> GHR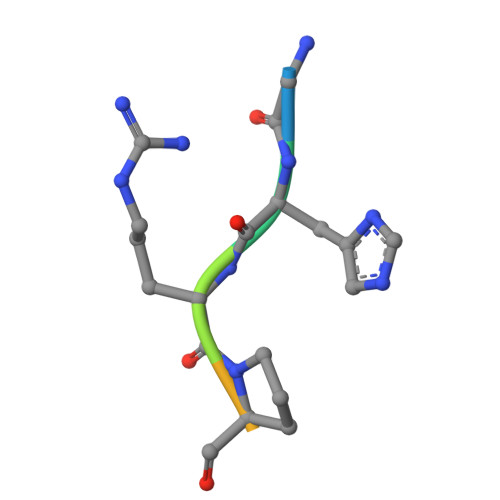PLDK> ETDICKLPKDEGTCRDFILKWYYDPNTK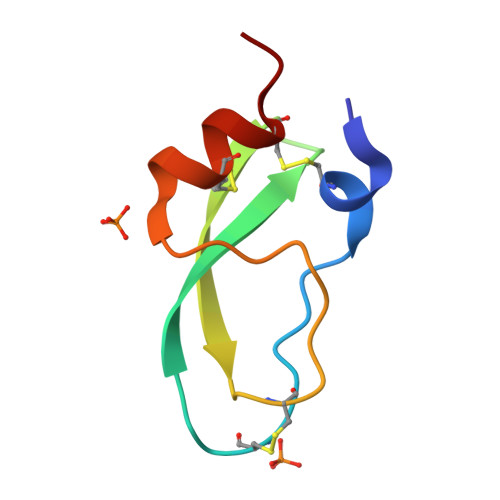SCARFWYGGCGGNENKFGSQKECEKVCAPV>SPNIKIFSGSSHQDLSQKIADRLGLELGKVVTKKFSNQETCVEIGESVRGEDVYIVQSGCGEINDNLMELLIMINACKIASASRVTAVIPCFPYARQDKKDKSRAPISAKLVANMLSVAGADHIITMDLHASQIQGFFDIPVDNLYAEPAVLKWIRENISEWRNCTIVSPDAGGAKRVTSIADRLNVDFALIHKERKKANEVDRMVLVGDVKDRVAILVDDMADTCGTICHAADKLLSAGATRVYAILTHGIFS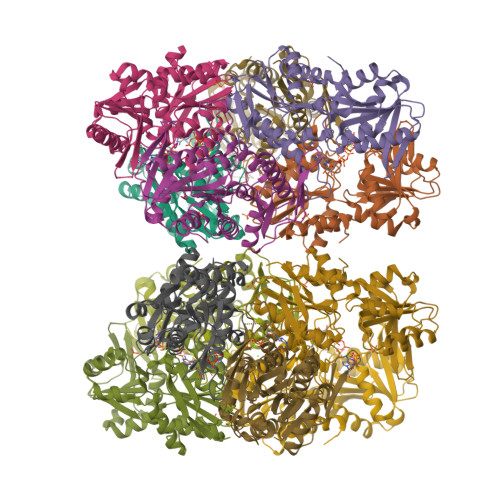GPAISRINNACFEAVVVTNTIPQEDKMKHCSKIQVIDISMILAEAIRRTHNGESVSYLFSHVPL[12x]> MGTLQKCFEDSNGKASDFSLEASVAEMKEYITKFSLERQTWDQLLLHYQQEAKEILSRGSTEAKITEVKVEPMTYLG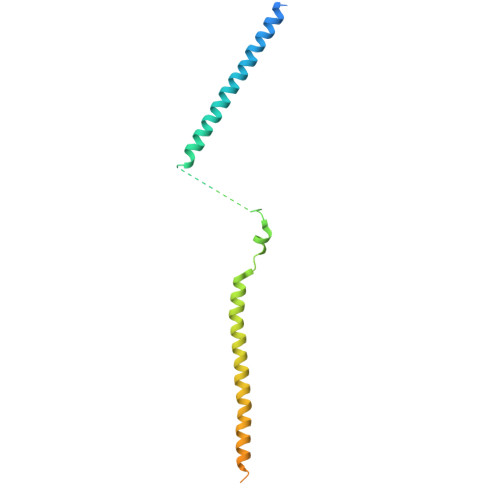SSQNEVLNTKPDYQKILQNQSKVFDCMELVMDELQGSVKQLQAFMDESTQCFQKVSVQLGKRSMQQLDPSPARKLLKLQLQNPPAIHGSGSGSCQHHHHHH>[2x]KPGAPWWKSAVFYQVYPRSFKDTNGDGIGDFKGLTEKLDYLKGLGIDAIWINPHYASPNTDNGYDISDYREVMKEYGTMEDFDRLMAELKKRGMRLMVDVVINHSSDQHEWFKSSRASKDNPYRDYYFWRDGKDGHEPNNYPSFFGGSAWEKDPVTGQYYLHYFGRQQPDLNWDTPKLREELYAMLRFWLDKGVSGMRFDTVATYSKTPGFPDLTPEQMKNFAEAYTQGPNLHRYLQEMHEKVFDHYDAVTAGEIFGAPLNQVPLFIDSRRKELDMAFTFDLIRYDRALDRWHTIPRTLADFRQTIDKVDAIAGEYGWNTFFLGNHDNPRAVSHFGDDRPQWREASAKALATVTLTQRGTPFIFQGDELGMTNYPFKTLQDFDDIEVKGFFQDY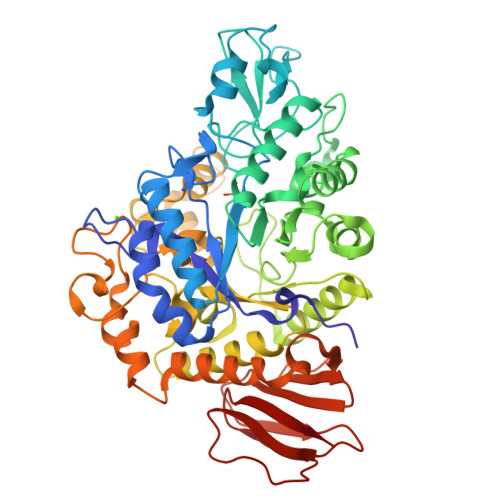VETGKATAEELLTNVALTSRDNARTPFQWDDSANAGFTTGKPWLKVNPNYTEINAAREIGDPKSVYSFYRNLISIRHETPALSTGSYRDIDPSNADVYAYTRSQDGETYLVVVNFKAEPRSFTLPDGMHIAETLIESSSPAAPAAGAASLELQPWQSGIYKVK>[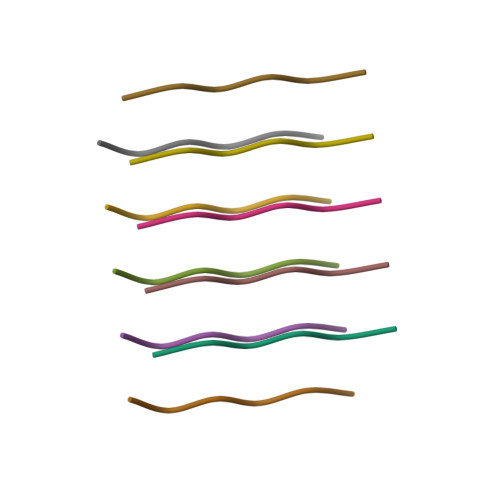2x]SVQIVY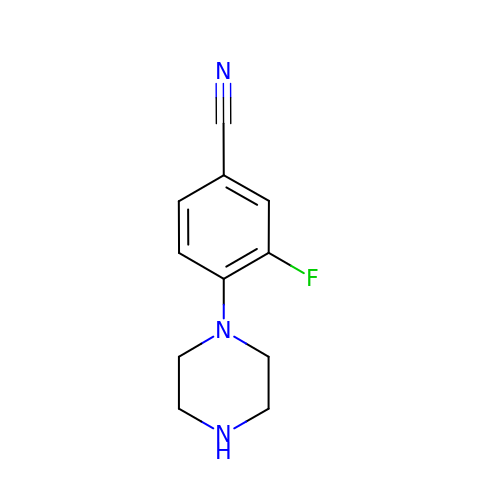3-fluoro-4-(piperazin-1-yl)benzonitrile | C11 H12 F N3 | VMOBEAUQUPPPON-UHFFFAOYSA-N>[2x]VCPNIIKRSAWEARETHCPKMNLPAKYVIIIHTAGTSCTVSTDCQTVVRNIQSFHMDTRNFCDIGYHFLVGQ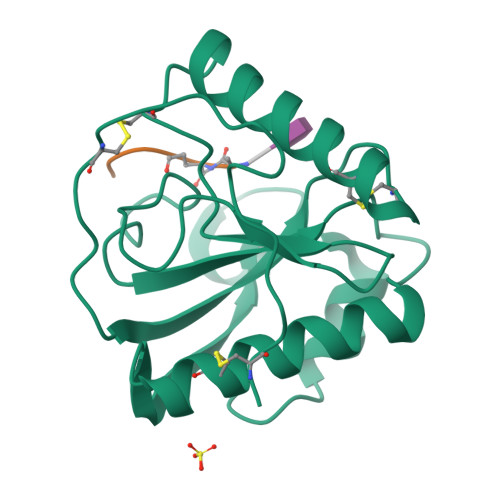DGGVYEGVGWHIQGSHTYGFNDIALGIAFIGYFVEKPPNAAALEAAQDLIQCAVVEGYLTPNYLLMGHSDVVNILSPGQALYNIISTWPHFKH;>[2x]AEKAAX>MTPLNPTDQLFLWLEKRQQPMHVGGLQLFSFPEGAPDDYVAQLADQLRQKTEVTAPFNQRLSYRLGQPVWVEDEHLDLEHHFRFEALPTPGRIRELLSFVSAEHSHLMDRERPMWEVHLIEGLKDRQFALYTKVHHSLVDGVSAMRMATRMLSENPDEHGMPPIWDLPCLSRDRGESDGHSLWRSVTHLLGLSGRQLGTIPTVAKELLKTINQARKDPAYDSIFHAPRCMLNQKITGSRRFAAQSWCLKRIRAVCEAYGTTVNDVVTAMCAAALRTYLMNQDALPEKPLVAFVPVSLRRDDSSGGNQVGVILASLHTDVQEAGERLLKIHHGMEEAKQRYRHMSPEEIVNYTALTLAPAAFHLLTGLAPKWQTFNVVISNVPGPSRPLYWNGAKLEGMYPVSIDMDRLALNMTLTSYNDQVEFGLIGCRRTLPSLQRMLDYLEQGLAELELNA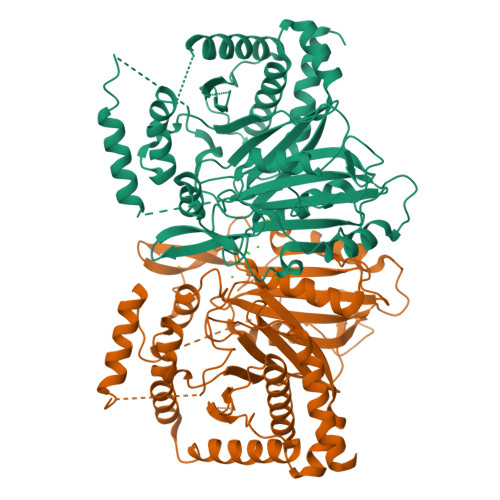GL[2x]The ParABS system, composed of ParA (an ATPase), ParB (a DNA binding protein), and parS (a centromere-like DNA), regulates bacterial chromosome partition. In Helicobacter pylori, ParA and ParB homologs are encoded as HpSoj and HpSpo0J (HpParA and HpParB), respectively. ParA forms as a dimer in the ATP-bound state that can bind to nsDNA through a continuous basic binding patch formed by arginine/lysine residues. The partition complex interacts with the nucleoid-bound ParA forming the nucleoprotein ParA–ParB–DNA complex, known as the nucleoid–adaptor complex (NAC).

In HpParA-DNA structures, four lysine residues, Lys199, Lys227, Lys230 and Lys247, have been reported to be involved in non-specific DNA binding, with Lys199 and Lys230 directly binding to DNA. In the HpParAD41A-DNA complex, an additional interaction with DNA involving Lys227 was observed. This conserved Lys227 residue is positioned at the core of the DNA binding surface, between the DNA backbone (4.0 Å) and ATP (3.6 Å). Since HpParAD41A is deficient in ATP hydrolysis ability, Lys227 may interact with the DNA backbone, resulting in the loss of the connection between ATP and DNA binding. The HpParAD41A-DNA complex displays a higher resolution of 2.6 Å compared to that of the HpParA–ATP–DNA complex structure (3.4 Å). The ATP-hydrolysis deficient mutant HpParAD41A exhibits low ATP hydrolysis activity and remains in a dimeric state while preserving DNA binding. Therefore, the HpParAD41A–DNA complex may adopt a stable conformation with bound DNA than that of HpParA. The HpParA–DNA and HpParAD41A-DNA complexes share similar overall structures, featuring an ATP binding pocket and a readily exposed continuous basic DNA binding patch. Once the HpParAD41A-DNA complex is formed, it may maintain a more stable conformation than HpParA and undergo a steady interaction with the N-terminus of HpParB.

>[4x]MMSEIIAVANQKGGVGKTTTAVNLAASLAVHEKKILLIDFAPQANATSSLGFRRDKIDYDIYHVLIGRKQISQVILKTQMPFLDLVPSNLGLAGFEKTFYDSQDENKRGELMLKNALESVVGLYDYIIIDSPPALGPLTINSLSAAHSVIIPIQCEFFALEGTKLLLNTIRMLQKSTNPKLKIRGFLPTMHVPQLNLTKGVLAELFKYFDSEFFRDSATGEYIMIPKSVKLAESPSFGKPILLYDIKSNGSIAYQKLAQSILQG> MQTVNEMLRRAATRAPDHCALAVPA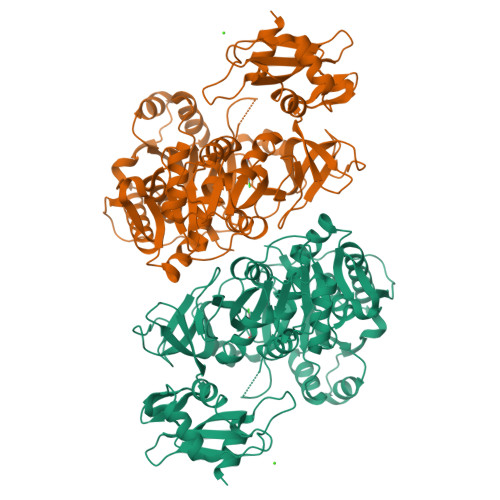RGLRLTHAELRARVEAVAARLHADGLRPQQRVAVVAPNSADVVIAILALHRLGAVPALLNPRLKSAELAELIKRGEMTAAVIAVGRQVADAIFQSGSGARIIFLGDLVRDGEPYSYGPPIEDPQREPAQPAFIFYTSGTTGLPKAAIIPQRAAESRVLFMSTQVGLRHGRHNVVLGLMPLYHVVGFFAVLVAALALDGTYVVVEEFRPVDALQLVQQEQVTSLFATPTHLDALAAAAAHAGSSLKLDSLRHVTFAGATMPDAVLETVHQHLPGEKVNIYGTTEAMNSLYMRQPKTGTEMAPGFFSEVRIVRIGGGVDEIVANGEEGELIVAASDSAFVGYLNQPQATAEKLQDGWYRTSDVAVWTPEGTVRILGRVDDMIISGGENIHPSEIERVLGTAPGVTEVVVIGLADQRWGQSVTACVVPRLGETLSADALDTFCRSSELADFKRPKRYFILDQLPKNALNKVLRRQLVQQVSS>MLEGDAKVAKILIAYASMSGNTESIADLIKVSLDAFDHEVVLQEMEGMDAEELLAYDGIILGSYTW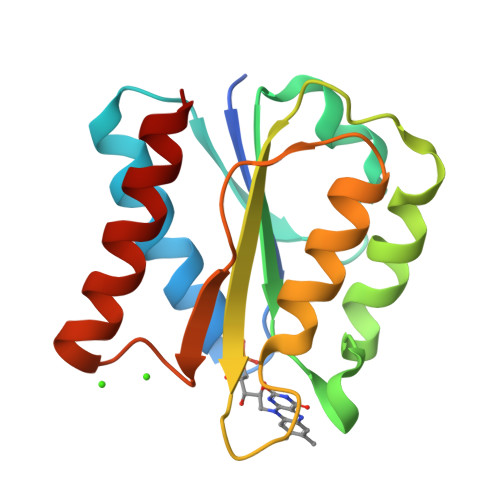GDGELPFEAEDFHDDLENIDLAGKKVAVFGSGDTAYELFCEAVTIFEERLVERGAELVQEGLKIELAPEDEEDVEKCSNFAIAFAEKF[2x]> KET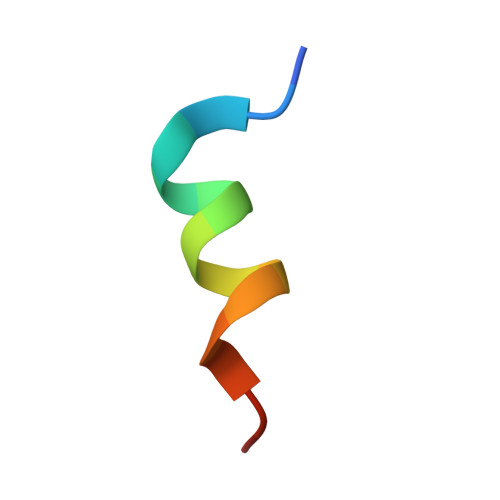AAAKFERQHMDSX A major factor that limits the expansion of shrimp cultures is, however, infectious diseases from viruses, such as P. vannamei nodavirus (PvNV) and M. rosenbergii nodavirus (MrNV), which have inflicted heavy economic losses. The Nodaviridae genome comprises two single-stranded positive-sense RNA that encode the capsid protein for viral capsid assembly, the RNA polymerase for RNA replication, and the B2 protein for host RNA interference suppressor. While the shell domains (S-domains) of PvNV and MrNV contain conserved sequences of 62% identity, the protrusion domains (P-domains) and N-arms show low sequence identities of only 17% and 43%, respectively. In this work, we have determined the cryo-EM structures of T = 3 and T = 1 PvNV-LPs at atomic resolution, the crystal structures of the P-domains of PvNV and MrNV (PvNVPd and MrNVPd), and the crystal structure of the S-domain of PvNV (ΔN-ARM-PvNVSd) in the T = 1 subviral particle (SVP).

As for the MrNvPd, three crystal forms (P3221, C2221, and P4332) were determined. The overall conformations and dimer interfaces in three crystal structures of MrNVPd are similar with a RMSD < 0.3 Å. The MrNVPd has a structural fold consisting of eight long stretches of antiparallel β-strands similar to the PvNVPd, but shares a low sequence homology with PvNVPd. In addition, the MrNVPd dimer is stabilized with hydrogen bonds between Leu255 and Tyr257 of the β1 strand and Lys287 and Ile289 of the β3 strand. Second, two MrNVPd dimers (C2221) in an asymmetric unit form an X-shaped model with the antiparallel β-strand interaction through an extensive network of hydrogen bonds between residues from two β-strands β2 (Gln273–Asp278) and two turns β1/β2 (Val266–Pro267). The two dimers in the X-shaped model are orientated with a tilt angle of 130° and with separation of ~63 Å between the two linker terminals. Notably, the sequence of the interaction region (Gln273–Asp278) of MrNVPd is distinct from that of PvNVPd, and two types (P21 and P212121) of PVNVPd structures do not exhibit the X-shaped conformation. It appears that the X-shaped dimeric MrNVPd organization reveals no homology compared with intermolecular P-domain conformations of other viral capsids. Although the X-shaped model is observed only in the MrNVPd structure, we speculate that this organization might both exist also on the T = 3 MrNV and PvNV virions under various environment even high salt or low pH.

>PTPVEVSQLTYNADTIGNWVPPTELKQTYTQDITGLKPNSKFIIVPYMDRVSSEVLQKCTITCNEVDAVGSISYFDTSAIKCDGYISFQANSIGEATFTLVTDYQGAVDPKPYQYRIIRAIVGNN[8x]>[2x]G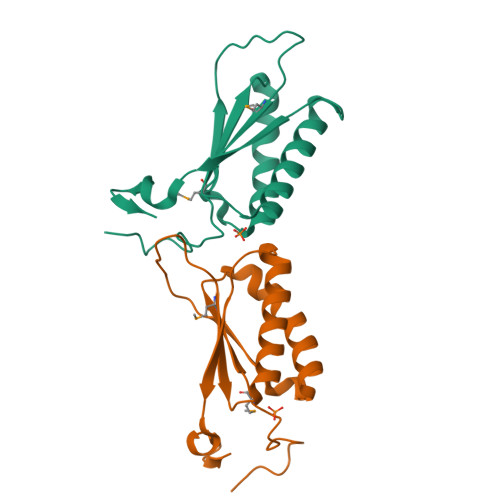VDLGTENLYFSSNAMPHLRFRAVEAHIVESLVPTLLNELSSLLSTARNAFTFELINTQYFAEGGVYPMVEVLWFGREQQTQDQIAQVITDQIRQLLGADSHLAVVFIPLQRTAYYLDGQHF>QRCGEQGSGMECPNNLCCSQYGYCGMGGDYCGKGCQNGACWTSKRCGSQAGGKTCPNNHCCSQYGHCGFGAEYCGAGCQGGPCRADIKCGSQAGGKLCPNNLCCSQWGYCGLGSEFCGEGCQNGACSTDKPCGKDAGGR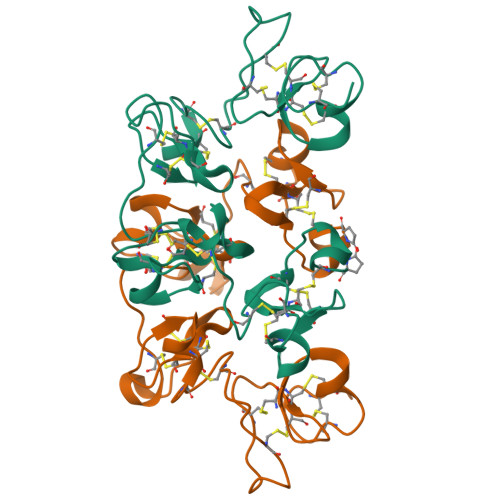VCTNNYCCSKWGSCGIGPGYCGAGCQSGGCDGVFAEAIATNSTLLAE[2x]> MERKISRIHLVSEPSITHFLQVSWEKTLESGFVITLTDGHSAWTGTVSESEISQ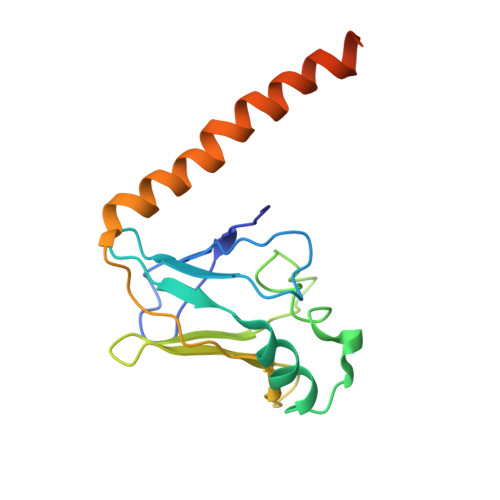EADDMAMEKGKYVGELRKALLSGAGPADVYTFNFSKESCYFFFEKNLKDVSFRLGSFNLEKVENPAEVIRELICYCLDTIAENQAKNEHLQKENERLLRDWNDHHHHHH> MGSSHHHHHHSSENLYFQGHKRIYVSYGSPVIDGEVDDIWNNVEWNIPRIYSATTQTNAKFKLMWDDNALYVLAEVYDPVLNSANSTPYQQDSVEIFLDENFDRAISYQSDDLHYRVNYNNFKTTDAGDILRFYTKTKLLPDGYRVEARIALSKKPINGTIMGFEFQVNEADSSARRVATINMFDNTGNAWQNPSLFGEIKLKGRSDNAVVPINP

The hyperthermophilic bacterium Caldicellulosiruptor kristjansonii encodes an unusual enzyme, CkXyn10C-GE15A, which incorporates two catalytic domains, a xylanase and a glucuronoyl esterase, and five carbohydrate-binding modules (CBMs) from families 9 and 22. C. kristjansonii has been shown to grow on a variety of polysaccharides, including cellulose, xylan, starch, and pectin, with an optimal growth temperature of 78 °C. From the N-terminus, CkXyn10C-GE15A consists of two CBM22 domains (CBM22.1 and CBM22.2), a GH10 endo-xylanase (Xyn10C), three CBM9 domains (CBM9.1, CBM9.2, and CBM9.3), a GE from CE15 (GE15A), a cadherin domain, and two surface layer homology (SLH) domains believed to anchor the protein to the Gram-positive cell wall. Collectively, the results show that all five CBMs have their own distinct binding preferences and appear to complement each other and the catalytic domains in targeting complex cell wall polysaccharides. We have determined the structures of the third CBM9 domain (CBM9.3) and the glucuronoyl esterase (GE15A) by X-ray crystallography.

To gain a deeper insight into the molecular determinants for carbohydrate binding of CBM9.3, we determined the structure using X-ray crystallography. Residue numbers in this section reflect the numbering of the PDB file, where Lys21 corresponds to Lys1071 in the full-length CkGE15A-Xyn10C protein sequence. The putative sugar-binding site was easily identifiable from comparisons with TmCBM9-2, and in CBM9.3, it is formed by the aromatic residues Tyr89, located on α-helix 2 between β-strands 4 and 5, and Trp191, located on a loop between β-strand 11 and α-helix 4. These contrast the dual tryptophan residues forming the sugar-binding clamp in TmCBM9-2 (Trp71 and Trp175), though the ability of CBM9.3 to bind various carbohydrates suggests this does not have a negative effect on the carbohydrate recognition for the protein. CBM9.3 shows metal-binding sites for the three calcium ions similar to those of TmCBM9-2, although the calcium ion near the loop between β-strands 4 and 5 in CBM9.3 is present at only approximately 50% occupancy. Additionally, although the overall structure of CBM9.3 is very similar to that of TmCBM9-2, the binding site appears to be much more open in CBM9.3 compared to a pocketlike site in TmCBM9-2. In TmCBM9-2, the binding site is blocked at one end by Asn172, with the equivalently positioned residue in CBM9.3 being Gly188 that, due to its small size, does not enclose the binding site. The C-terminal linker region included in the construct is observed as an extended tail seen in CBM9.3. This tail closely interacts with the tail in a symmetry-related protein molecule, along with the protein surface near the tail of this symmetry-related protein molecule.>[2x]TGFDFNAYMGEKAAAVNRALDASIPADEPPAALHEAMRYALLAGGKRVRPALCLAACAVVGGREAWAMPAAAAVEMVHTMSLVHDDLPCMDDDDLRRGKPTCHVVYGEPIAVLTGDALLSLSFHHMARFDSYPPDIDADKHPARVVRAIGELARCIGSEGLVAGQVVDLEMTGSTETVPLERLEYIHLHKTAALLEASVVIGAILGGGSDEQIESLRMYARSIG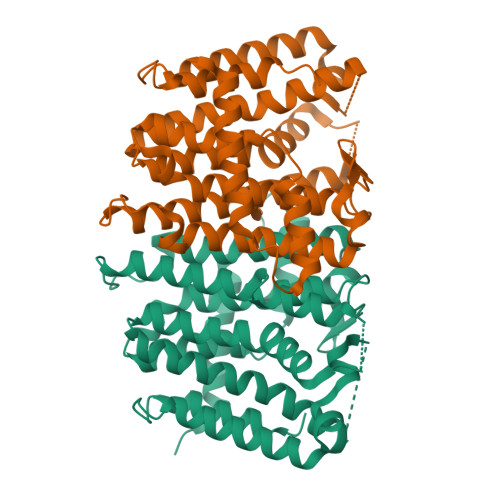LLFQVVDDILDVTKSSEELGKTAGKDLASDKTTYPKLLGLEKSREFAEKLLSDAREQLSGFDQETAAPLLHLANYIAYRQN> TGLAADIRWTAYGVPHIRAKDERGLGYGIGYAYARDNACLLAEEIVTARGERARYFGSEGKSSAELDNLPSDIFYAWLNQPEALQAFWQAQTPAVRQLLEGYAAGFNRFLREADGKTTSCLGQPWLRAIATDDLLRLTRRLLVEGGVGQFADALVAAAPPGAE;> SNAIAVGSERSADGKGMLLANPHFPWNGAMRFYQMHLTIPGRLDVMGASLPGLPVVNIGFSRHLAWTHTVDTSSHFTLYRLALDPKDPRRYLVDGRSLPLEEKSVAIEVRGADGKLSRVEHKVYQSIYGPLVVWPGKLDWNRSEAYALRDANLENTRVLQQWYSINQASDVADLRRRVEALQGIPWVNTLAADEQGNALYMNQSVVPYLKPELIPACAIPQLVAEGLPALQGQDSRCAWSRDPAAAQAGITPAAQLPVLLRRDFVQNSND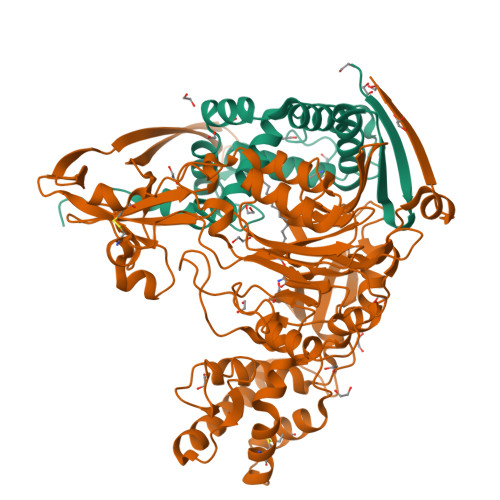SAWLTNPASPLQGFSPLVSQEKPIGPRARYALSRLQGKQPLEAKTLEEMVTANHVFSADQVLPDLLRLCRDNQGEKSLARACAALAQWDRGANLDSGSGFVYFQRFMQRFAELDGAWKEPFDAQRPLDTPQGIALDRPQVATQVRQALADAAAEVEKSGIPDGARWGDLQVSTRGQERIAIPGGDGHFGVYNAIQSVRKGDHLEVVGGTSYIQLVTFPEEGPKARGLLAFSQSSDPRSPHYRDQTELFSRQQWQTLPFSDRQIDADPQLQRLSIRE(3~{R},4~{R},5~{S})-4-acetamido-5-[4-(hydroxymethyl)-1,2,3-triazol-1-yl]-3-pentan-3-yloxy-cyclohexene-1-carboxylic acid | C17 H26 N4 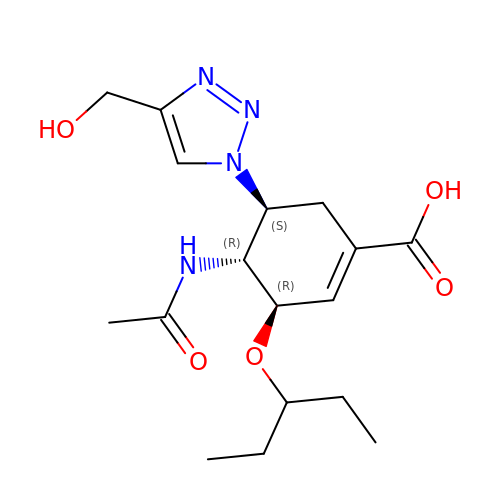O5 | IPVDZUUVRPUAMB-ARFHVFGLSA-N>[2x]MAHHHHHHMASPASTNPAHDHFETFVQAQLCQDVLSSFQGLCRALGVESGGGLSQYHKIKAQLNYWSAKSLWAKLDKRASQPVYQQGQACTNTKCLVVGAGPCGLRAAVELALLGA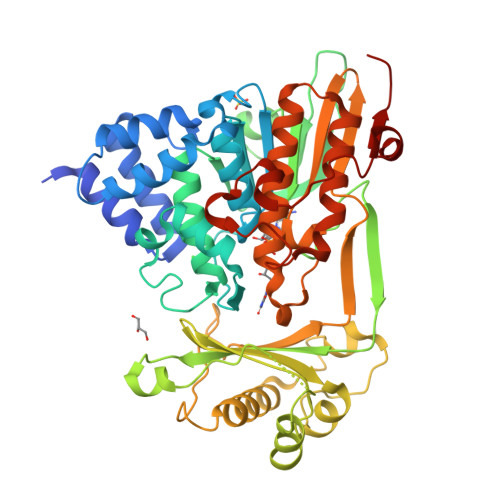RVVLVEKRIKFSRHNVLHLWPFTIHDLRALGAKKFYGRFCTGTLDHISIRQLQLLLLKVALLLGVEIHWGVKFTGLQPPPRKGSGWRAQLQPNPPAQLASYEFDVLISAAGGKFVPEGFTIREMRGKLAIGITANFVNGRTVEETQVPEISGVARIYNQKFFQSLLKATGIDLENIVYYKDETHYFVMTAKKQCLLRLGVLRQDLSETDQLLGKANVVPEALQRFARAAADFATHGKLGKLEFAQDARGRPDVAAFDFTSMMRAESSARVQEKHGARLLLGLVGDCLVEPFWPLGTGVARGFLAAFDAAWMVKRWAEGAGPLEVLAERESLYQLLSQTSPENMHRNVAQYGLDPATRYPNLNLRAVTPNQVQDLYDMMDKE>[2x]SVKLAGNSSLCPVSGWAIYSKDNSVRIGSKGDVFVIREPFISCSPLECRTFFLTQGALLNDKHSNGTIKDRSPYRTLMSCPIGEV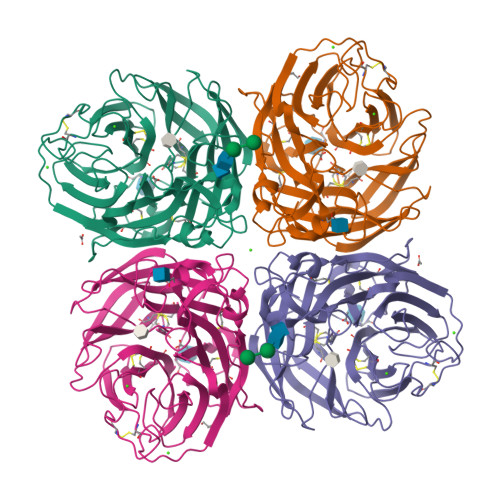PSPYNSRFESVAWSASACHDGINWLTIGISGPDNGAVAVLKYNGIITDTIKSWRNNILRTQESECACVNGSCFTVMTDGPSNGQASYKIFRIEKGKIVKSVEMNAPNYHYEECSCYPDSSEITCVCRDNWHGSNRPWVSFNQNLEYQIGYICSGIFGDNPRPNDKTGSCGPVSSNGANGVKGFSFKYGNGVWIGRTKSISSRNGFEMIWDPNGWTGTDNNFSIKQDIVGINEWSGYSGSFVQHPELTGLDCIRPCFWVELIRGRPKENTIWTSGSSISFCGVNSDTVGWSWPDGAELPFTIDK>GCG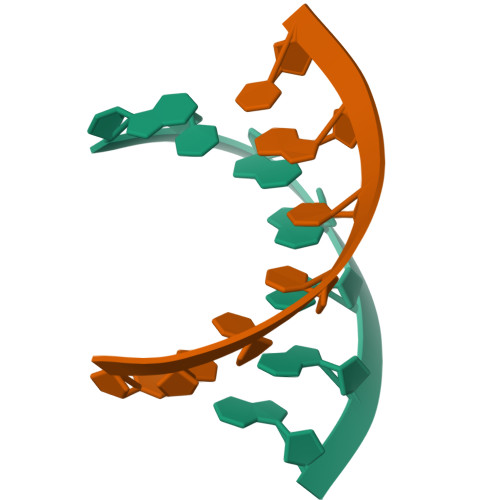GGAG[2x];>CUCCCGC[2x]> 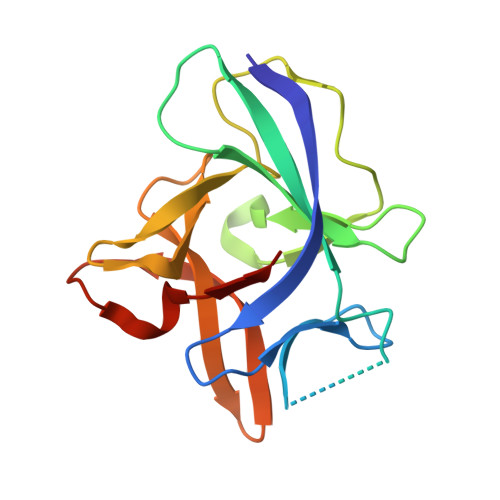YFGKLESKLSVIRNLNDQVLFIDQGNRPLFEDMTDSDSRDNAPRTIFIISMYKDSQPRGMAVTISVASAAASTLSSENKIISFKEMNPPDNIKDTKSDIIFFQRSVPGHDNKMQFESSSYEGYFLASEKERDLFKLILKKEDELGDRSIMFTVQNED> GEVASVPLTNYLDSQYFGKIYLGTPPQEFTVLFDTGSSDFWVPSIYCKSNACKNHQRFDPRKSSTFQNLGKPLSIHYGTGSMQGILGYDTVTVSNIVDIQQTVGLSTQEPGDFFTYAEFDGILGMAYPSLASEYSIPVFDNMMNRHLVAQDLFSVYMDRNGQESMLTLGAIDPS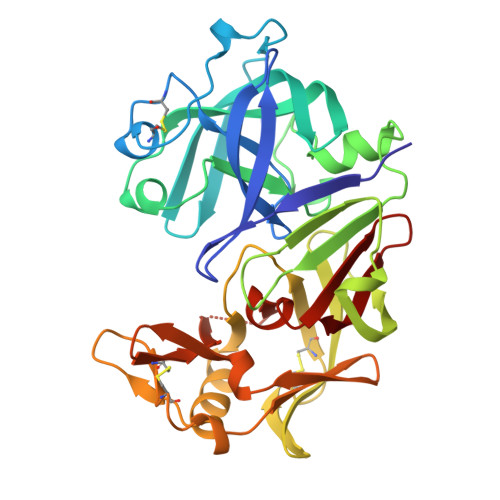YYTGSLHWVPVTVQQYWQFTVDSVTISGVVVACEGGCQAILDTGTSKLVGPSSDILNIQQAIGATQNQYGEFDIDCDNLSYMPTVVFEINGKMYPLTPSAYTSQDQGFCTSGFQSENHSQKWILGDVFIREYYSVFDRANNLVGLAKAI>[52x]MNNLYRDLAPVTEAAWAEIELEAARTFKRHIAGRRVVDVSDPGGPVTAAVSTGRLIDVKAPTNGVIAHLRASKPLVRLRVPFTLSRNEIDDVERGSKDSDW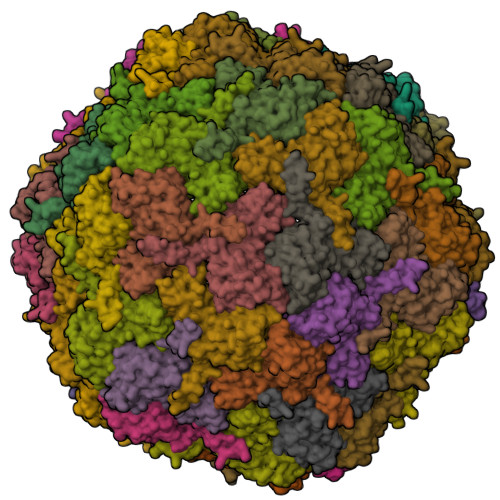EPVKEAAKKLAFVEDRTIFEGYSAASIEGIRSASSNPALTLPEDPREIPDVISQALSELRLAGVDGPYSVLLSADVYTKVSETSDHGYPIREHLNRLVDGDIIWAPAIDGAFVLTTRGGDFDLQLGTDVAIGYASHDTDTVRLYLQETLTFLCYTAEASVALSH3-[3-({[3-(4-carboxyphenoxy)phenyl]methoxy}methyl)phenyl]-1H-indole-2-carboxylic acid | C30 H23 N O6 | 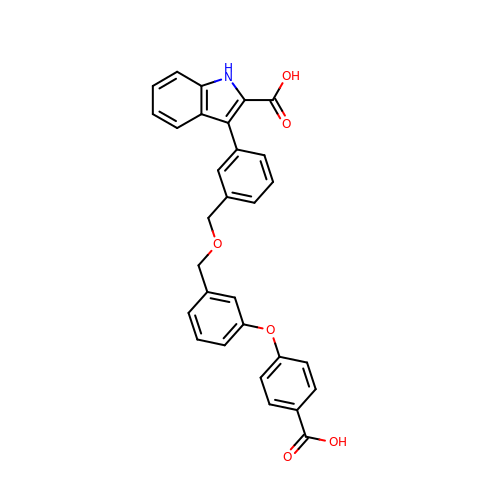LURNKRQADJFMRR-UHFFFAOYSA-N> TEDEIRKLRKLLEEAEKKLYKLEDKTRRSEEISKTDDDPKAQSLQLIAESLMLIAESLLIIAISL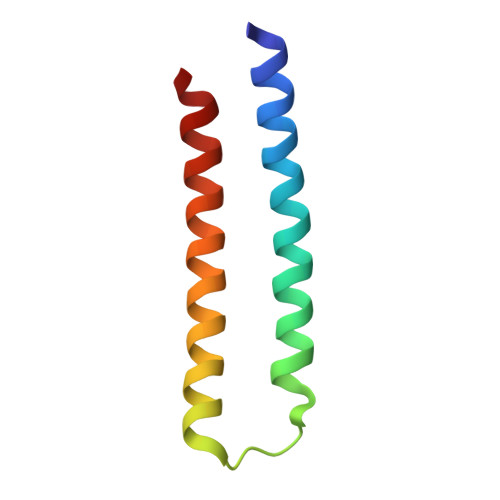LLSS>[8x]MHNDKDLSTWQTFRRLWPTIAPFKAGLIVAGVALILNAASDTFMLSLLKPLLDDGFGKTDRSVLVWMPLVVIGLMILRGITSYVSSYCISWVSGKVVMTMRRRLFG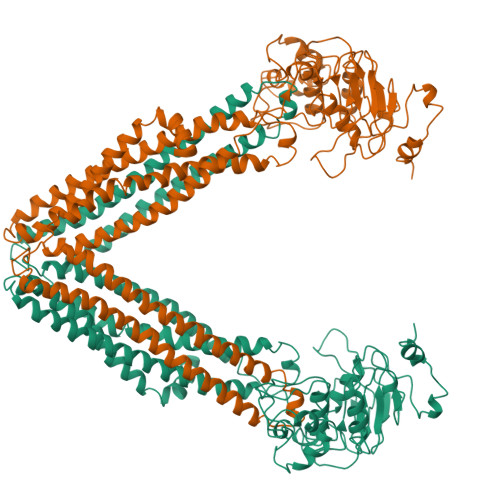HMMGMPVSFFDKQSTGTLLSRITYDSEQVASSSSGALITVVREGASIIGLFIMMFYYSWQLSIILIVLAPIVSIAIRVVSKRFRNISKNMQNTMGQVTTSAEQMLKGHKEVLIFGGQEVETKRFDKVSNRMRLQGMKMVSASSISDPIIQLIASLALAFVLYAASFPSVMDSLTAGTITVVFSSMIALMRPLKSLTNVNAQFQRGMAACQTLFTILDSEQEKDEGKRVIERATGDVEFRNVTFTYPGRDVPALRNINLKIPAGKTVALVGRSGSGKSTIASLITRFYDIDEGEILMDGHDLREYTLASLRNQVALVSQNVHLFNDTVANNIAYARTEQYSREQIEEAARMAYAMDFINKMDNGLDTVIGENGVLLSGGQRQRIAIARALLRDSPILILDEATSALDTESERAIQAALDELQKNRTSLVIAHRLSTIEKADEIVVVEDGVIVERGTHNDLLEHRGVYAQLHKMQFGQ> PA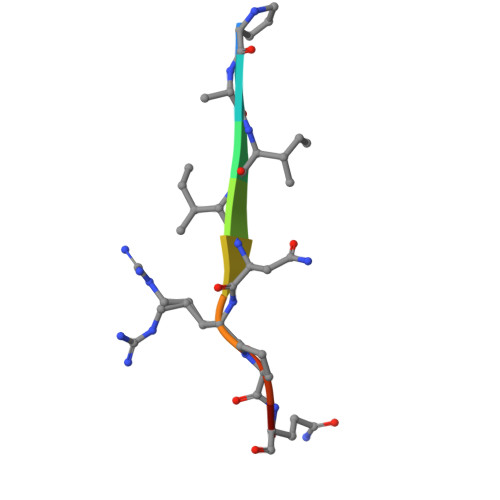IINRPQN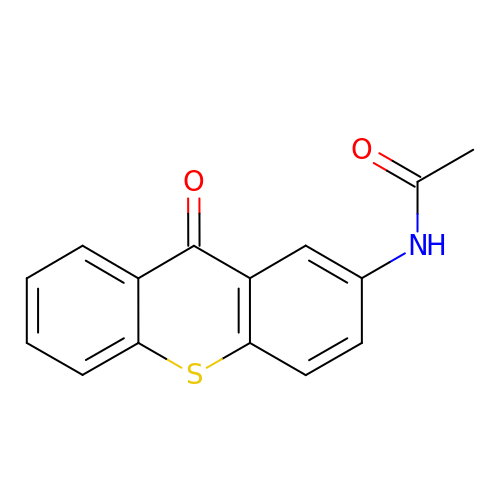N-(9-oxidanylidenethioxanthen-2-yl)ethanamide | C15 H11 N O2 S | GLOTXRJEKGIJGO-UHFFFAOYSA-N>MIRIPKSEYARRRKALMAQMEPNSIAILPAAPMYIRNRDVEHVYRQDSDFQYLTGFPEPEAVMALIPGRAHGEYVLFCRERDPERELWDGLRAGQDGAIGQYGADDAFPIGDIDDILPGLIEGRDRVYYALGANPDFDRRLMDWINVIRSKARQGAQPPNEFVALDHLLHDQRLYKSANEVKVMRYAAEVSARAHIRAMEVCRPGLFEYHLEAELEYEFRKGGAKMPAYGSIVAAGRNACILHYRENDAAIKDGDLILIDAGCEIDCYASDITRTFPANGRFSPEQKAIYELVLEANMAAFDYIAPGRHWNEAHEATVRVITAGLVRLGLLEGDVDELIAHEAYKAFYMHRAGHWLGMDVHDVGEYRVGGEWRVLEPGMAMTVEPGIYIAPDNTTVAKKWRGIGVRIEDDVVVTRNGCEVLTNGVPKTVAEIEALMAAAKSEAALEHH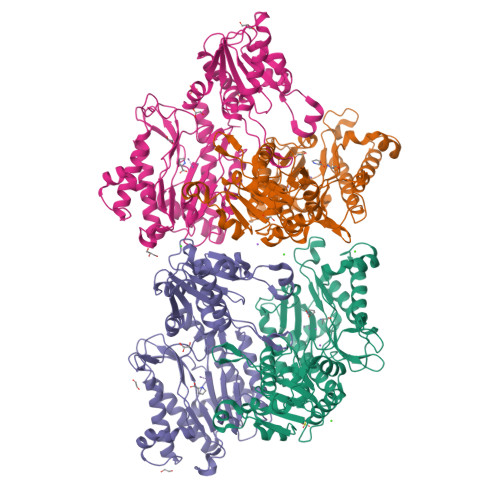HHHH[4x]>MNHKVHHHHHHIEGRHMPFEIVFDGAKEFADLIATASNLIDEAAFKITEEGVSMRAMDPSRVVLIDLNLPES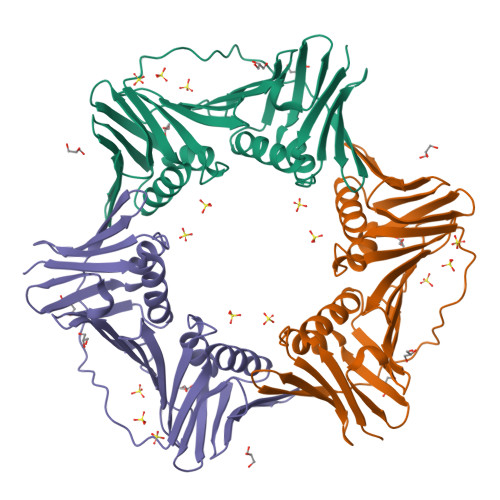IFSKYEVEEPETIGINMDHFKKILKRGKSKDTLILRKGDENFLEITFEGTAKRTFRLPLIDVEELELELPELPFTAKVVLLGEVLKEAIKDASLVSDSLKFIAKEDEFTMKAEGETNEVEIKLTLEDEGLLDLEVEEETRSAYGISYLADMVKGIGKADEVTLRFGTEMPLQMDYFIRDEGKLTFLLAPRVEE[2x]> MPHRFKVYNYMSPTFCDHCGSLLWGLVKQGLKCEDCGMNVH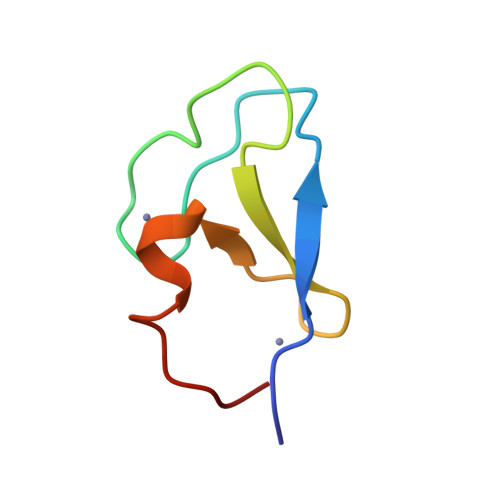HKCREKVANLCG>[2x]QRMK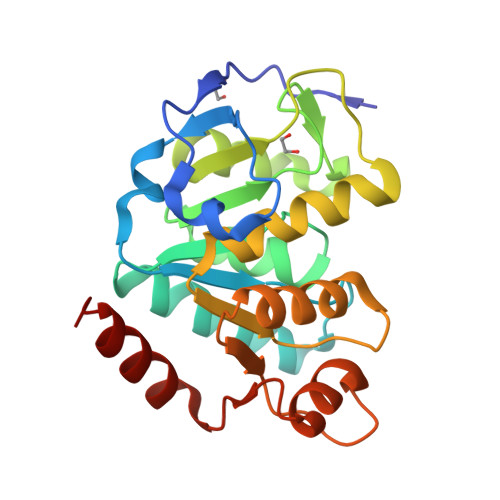SHFQYSTLENIPKAFDILKDPPKKLYCVGDTKLLDTPLKVAIIGTRRPTPYSKQHTITLARELAKNGAVIVSGGALGVDIIAQENALPKTIMLSPCSLDFIYPTNNHKVIQEIAQNGLILSEYEKDFMPIKGSFLARNRLVIALSDVVIIPQADLKSGSMSSARLAQKYQKPLFVLPQRLNESDGTNELLEKGQAQGIFNIQNFINTLLKDYHLK>[2x]MDAKFLEILVCPLCKGPLVFDKS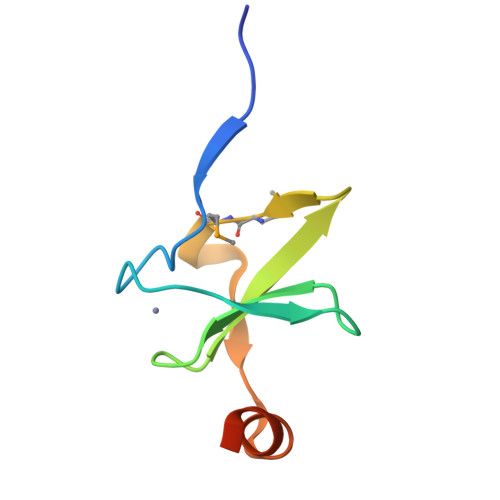KDELICKGDRLAFPIKDGIPMMLESEARELAPEEEVKLEHHHHHH>[2x]DAAP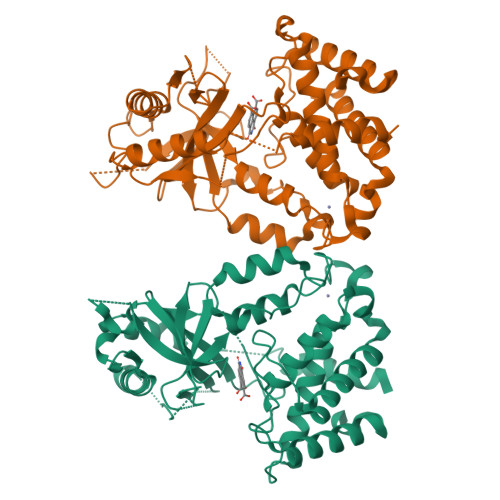GASKLRAVLEKLKLSRDDISTAAGMVKGVVDHLLLRLKCDSAFRGVGLLNTGSYYEHVKISAPNEFDVMFKLEVPRIQLEEYSNTRAYYFVKFKRNPKENPLSQFLEGEILSASKMLSKFRKIIKEEINDIKDTDVIMKRKRGGSPAVTLLISEKISVDITLALESKSSWPASTQEGLRIQNWLSAKVRKQLRLKPFYLVPKHAKEGNGFQEETWRLSFSHIEKEILNNHGKSKTCCENKEEKCCRKDCLKLMKYLLEQLKERFKDKKHLDKFSSYHVKTAFFHVCTQNPQDSQWDRKDLGLCFDNCVTYFLQCLRTEKLENYFIPEFNLFSSNLIDKRSKEFLTKQIEYERNNEFPVFDEF>[2x]ASLTEIEHLVQSVCKSYRETCQLRLEDLLRQRSNI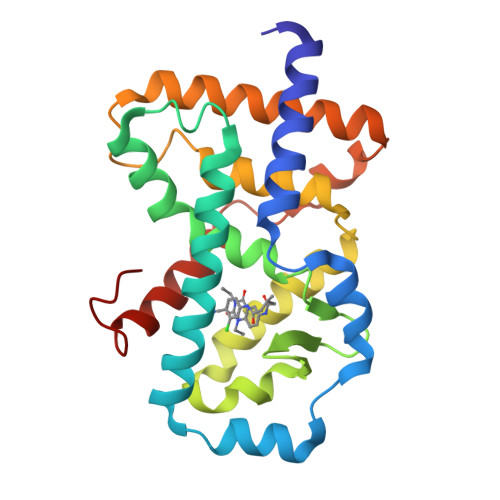FSREEVTGYQRKSMWEMWERCAHHLTEAIQYVVEFAKRLSGFMELCQNDQIVLLKAGAMEVVLVRMCRAYNADNRTVFFEGKYGGMELFRALGCSELISSIFDFSHSLSALHFSEDEIALYTALVLINAHRPGLQEKRKVEQLQYNLELAFHHHLCKTHRQSILAKLPPKGKLRSLCSQHVERLQIFQHLHPI>GTENLYFQSMDELLRRAVPPTPAYELRAATPAPAEGQCADFVSFYGGLAETAQRAELLGRLARGFGVDHGQVAEQSAGVLHLRQQQREAAVLLQAEDRLRYALVPRYRGLFHHISKLDGGVRFLVQLRADLLEAQALKLVEGPDVREMNGVLKGMLSEWFSSGFLNLERVTWHSPCEVLQKISEAEAVHPVKNWMDMKRRVGPYRRCYFFSHCSTPGEPLVVLHVALTGDISSNIQAIVKEHPPSETAAANKITAAIFYSISLTQQGLQGVELGTFLIKRVVKELQREFPHLGVFSSLSPIPGFTKWLLGLLNSQTKEHGRNELFTDSECKEISEITGGPINETLKLLLSSSEWVQSEKLVRALQTPLMRLCAWYLYGEKHRGYALNPVANFHLQNGAVLWRINWMADVSLRGITGSCGLMANYRYFLEETGPNSTSYLGSKIIKASEQVLSLVAQFQKN[2x]

Malonyl-coenzyme A decarboxylase (MCD) is found from bacteria to humans, has important roles in regulating fatty acid metabolism and food intake, and is an attractive target for drug discovery. The MCD monomer contains an N-terminal helical domain involved in oligomerization and a C-terminal catalytic domain. Unexpectedly, the MCD catalytic domain is structurally homologous to those of the GCN5-related N-acetyltransferase superfamily, especially the curacin A polyketide synthase catalytic module, with a conserved His-Ser/Thr dyad important for catalysis. The catalytic domain of MCD contains a central eight-stranded, mostly antiparallel β sheet (β1–β8) that is surrounded by at least 11 α helices (α1–α11).

Wild-type HsMCD (residues 40–491, corresponding to the mature mitochondrial form) failed to crystallize. The structure of the E58A/K59A/E278A/E279A/K280A quintuple mutant was determined by single isomorphous replacement with anomalous scattering and refined at 2.8 Å resolution. The mutant exhibited similar oligomeric and enzymatic properties as wild-type HsMCD. Inspection of the structure revealed both alanine-substituted patches to be located in surface-exposed regions: Glu58-Lys59 was found in the loop connecting helices αA and αB, while the loop containing residues 278–280, connecting strands β3 and β4, was disordered. HsMCD is a tetramer in solution based on gel filtration chromatography and analytical ultracentrifugation (AUC) studies, consistent with the reported oligomerization state of many purified MCD enzymes. The HsMCD crystal structure shows that the tetramer is made of a dimer of dimers. A tight dimer of HsMCD is formed by extensive contacts of the helical domains of the two monomers, and the αD and αE helical inserts of the two monomers interact with each other in this dimer interface. Two HsMCD dimers then associate with each other through their catalytic domains, at ∼60° angle for the planes of the two dimers, to form the tetramer with 222 symmetry. The S329A mutant of HsMCD had a 110-fold loss in kcat and 58-fold loss in kcat/Km, and the H423N mutant had a 7-fold loss in kcat, consistent with their important roles in catalysis. Using HsMCD as example, we postulate that MCD proceeds through the formation of the tautomerized enolate intermediate, with the Ser329 and His423 dyad adopting important catalytic roles consistent with our docking and kinetic analysis.> GGUUAAGCGACU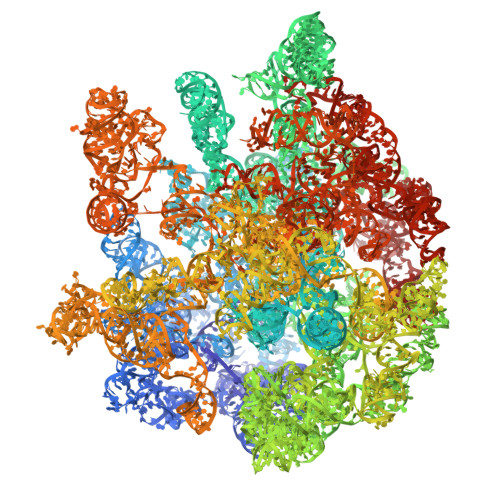AAGCGUACACGGUGGAUGCCCUGGCAGUCAGAGGCGAUGAAGGACGUGCUAAUCUGCGAUAAGCGUCGGUAAGGUGAUAUGAACCGUUAUAACCGGCGAUUUCCGAAUGGGGAAACCCAGUGUGUUUCGACACACUAUCAUUAACUGAAUCCAUAGGUUAAUGAGGCGAACCGGGGGAACUGAAACAUCUAAGUACCCCGAGGAAAAGAAAUCAACCGAGAUUCCCCCAGUAGCGGCGAGCGAACGGGGAGCAGCCCAGAGCCUGAAUCAGUGUGUGUGUUAGUGGAAGCGUCUGGAAAGGCGCGCGAUACAGGGUGACAGCCCCGUACACAAAAAUGCACAUGCUGUGAGCUCGAUGAGUAGGGCGGGACACGUGGUAUCCUGUCUGAAUAUGGGGGGACCAUCCUCCAAGGCUAAAUACUCCUGACUGACCGAUAGUGAACCAGUACCGUGAGGGAAAGGCGAAAAGAACCCCGGCGAGGGGAGUGAAAAAGAACCUGAAACCGUGUACGUACAAGCAGUGGGAGCACGCUUAGGCGUGUGACUGCGUACCUUUUGUAUAAUGGGUCAGCGACUUAUAUUCUGUAGCAAGGUUAACCGAAUAGGGGAGCCGAAGGGAAACCGAGUCUUAACUGGGCGUUAAGUUGCAGGGUAUAGACCCGAAACCCGGUGAUCUAGCCAUGGGCAGGUUGAAGGUUGGGUAACACUAACUGGAGGACCGAACCGACUAAUGUUGAAAAAUUAGCGGAUGACUUGUGGCUGGGGGUGAAAGGCCAAUCAAACCGGGAGAUAGCUGGUUCUCCCCGAAAGCUAUUUAGGUAGCGCCUCGUGAAUUCAUCUCCGGGGGUAGAGCACUGUUUCGGCAAGGGGGUCAUCCCGACUUACCAACCCGAUGCAAACUGCGAAUACCGGAGAAUGUUAUCACGGGAGACACACGGCGGGUGCUAACGUCCGUCGUGAAGAGGGAAACAACCCAGACCGCCAGCUAAGGUCCCAAAGUCAUGGUUAAGUGGGAAACGAUGUGGGAAGGCCCAGACAGCCAGGAUGUUGGCUUAGAAGCAGCCAUCAUUUAAAGAAAGCGUAAUAGCUCACUGGUCGAGUCGGCCUGCGCGGAAGAUGUAACGGGGCUAAACCAUGCACCGAAGCUGCGGCAGCGACGCUUAUGCGUUGUUGGGUAGGGGAGCGUUCUGUAAGCCUGCGAAGGUGUGCUGUGAGGCAUGCUGGAGGUAUCAGAAGUGCGAAUGCUGACAUAAGUAACGAUAAAGCGGGUGAAAAGCCCGCUCGCCGGAAGACCAAGGGUUCCUGUCCAACGUUAAUCGGGGCAGGGUGAGUCGACCCCUAAGGCGAGGCCGAAAGGCGUAGUCGAUGGGAAACAGGUUAAUAUUCCUGUACUUGGUGUUACUGCGAAGGGGGGACGCAGAAGGCUAUGUUGGCCGGGCGACGGUUGUCCCGGUUUAAGCGUGUAGGCUGGUUUUCCAGGCAAAUCCGGAAAAUCAAGGCUGAGGCGUGAUGACGAGGCACUACGGUGCUGAAGCAACAAAUGCCCUGCUUCCAGGAAAAGCCUCUAAGCAUCAGGUAACAUCAAAUCGUACCCCAAACCGACACAGGUGGUCAGGUAGAGAAUACCAAGGCGCUUGAGAGAACUCGGGUGAAGGAACUAGGCAAAAUGGUGCCGUAACUUCGGGAGAAGGCACGCUGAUAUGUAGGUGAGGUCCCUCGCGGAUGGAGCUGAAAUCAGUCGAAGAUACCAGCUGGCUGCAACUGUUUAUUAAAAACACAGCACUGUGCAAACACGAAAGUGGACGUAUACGGUGUGACGCCUGCCCGGUGCCGGAAGGUUAAUUGAUGGGGUUAGCGCAAGCGAAGCUCUUGAUCGAAGCCCCGGUAAACGGCGGCCGUAACUAUAACGGUCCUAAGGUAGCGAAAUUCCUUGUCGGGUAAGUUCCGACCUGCACGAAUGGCGUAAUGAUGGCCAGGCUGUCUCCACCCGAGACUCAGUGAAAUUGAACUCGCUGUGAAGAUGCAGUGUACCCGCGGCAAGACGGAAAGACCCCGUGAACCUUUACUAUAGCUUGACACUGAACAUUGAGCCUUGAUGUGUAGGAUAGGUGGGAGGCUUUGAAGUGUGGACGCCAGUCUGCAUGGAGCCGACCUUGAAAUACCACCCUUUAAUGUUUGAUGUUCUAACGUUGACCCGUAAUCCGGGUUGCGGACAGUGUCUGGUGGGUAGUUUGACUGGGGCGGUCUCCUCCUAAAGAGUAACGGAGGAGCACGAAGGUUGGCUAAUCCUGGUCGGACAUCAGGAGGUUAGUGCAAUGGCAUAAGCCAGCUUGACUGCGAGCGUGACGGCGCGAGCAGGUGCGAAAGCAGGUCAUAGUGAUCCGGUGGUUCUGAAUGGAAGGGCCAUCGCUCAACGGAUAAAAGGUACUCCGGGGAUAACAGGCUGAUACCGCCCAAGAGUUCAUAUCGACGGCGGUGUUUGGCACCUCGAUGUCGGCUCAUCACAUCCUGGGGCUGAAGUAGGUCCCAAGGGUAUGGCUGUUCGCCAUUUAAAGUGGUACGCGAGCUGGGUUUAGAACGUCGUGAGACAGUUCGGUCCCUAUCUGCCGUGGGCGCUGGAGAACUGAGGGGGGCUGCUCCUAGUACGAGAGGACCGGAGUGGACGCAUCACUGGUGUUCGGGUUGUCAUGCCAAUGGCACUGCCCGGUAGCUAAAUGCGGAAGAGAUAAGUGCUGAAAGCAUCUAAGCACGAAACUUGCCCCGAGAUGAGUUCUCCCUGACCCUUUAAGGGUCCUGAAGGAACGUUGAAGACGACGACGUUGAUAGGCCGGGUGUGUAAGCGCAGCGAUGCGUUGAGCUAACCGGUACUAAUGAACCGUGAGGCUUAACCUU>[2x]MVSKGEEDNMASLPATHELHIFGSINGVDFDMVGQGSGNPNVGYEELNLKSTKGDLQFSPWILVPHIGYGFHQYLPYPDGMSPFQAAMVDGSGYQVHRTVQFEDGASLTVNYRYTYEGSHIKGEAQVKGTGFPADGPVMANSLTAMVPSEEELSECFRTFDKDGDGFIDREEFGGIIRLTGEQLTDEDPDEIFGDSDTDKNGRID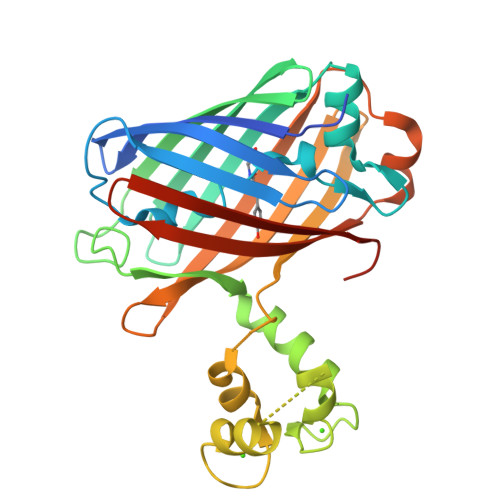FDEFLKMVENVQLSMADWCRSKMACPNDKTLISTLKWSYTTGNGKRYRSTARTTYTFAKPMAANYLKNQPMYVFRKTELKHSKTELNFKEWQKAFTDVMGMDELYK>MGKKMVVALGGNAILSNDASAHAQQQALVQTSAYLVHLIKQGHRLIVSHGNGPQVGNLLLQQQAADSEKNPAMPLDTCVAMTQGSIGYWLSNALNQELNKAGIKKQVATVLTQVVVDPADEAFKNPTKPIGPFLTEAEAKEAMQAGAIFKEDAGRGWRKVVPSPKPIDIHEAETINTLIKNDIITISCGGGGIPVVGQELKGVEAVIDKDFASEKLAELVDADALVILTGVDYVCINYGKPDEKQLTNVTVAELEEYKQAGHFAPGSMLPKIEAAIQFVESQPNKQAIITSLENLGSMSGDEIVGT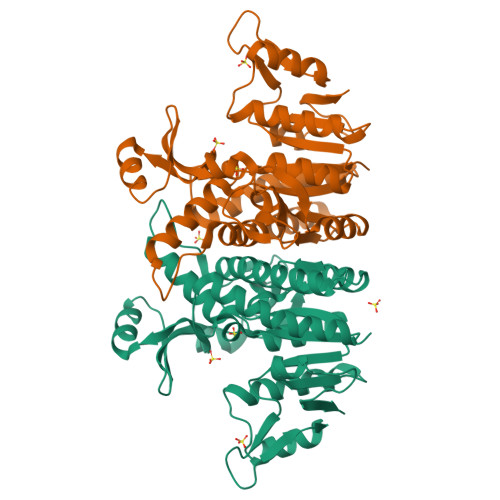VVTK[4x]>[4x]GHMTPTLETKYVFTITARIGDVTSAGEIGTGVRRIIPILGGEVKGEGISGQVLPFGADFQIIRPNELIELEAKYAFETDDGAV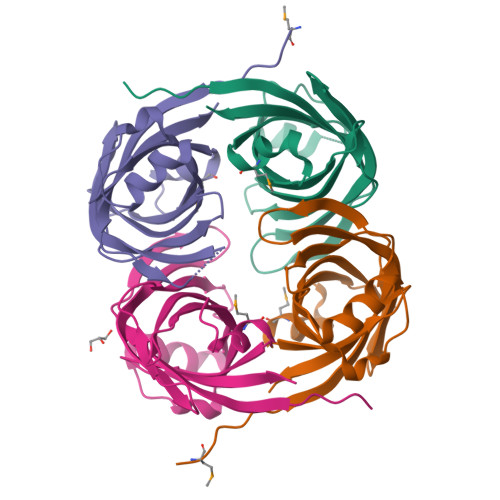VYVENVGIRFGPVELLRKLKRGEPVDPKVIYFRTRPRFETGHPNYQWLMQYLFVGSAARHADRVVIDVHQVLGS> TELTKCKVSHAIKDIDGYQGISLLEWACVLFHTSGYDTQAVVNDNGSTEYGLFQISDRFWCKSSEFPESENICGIS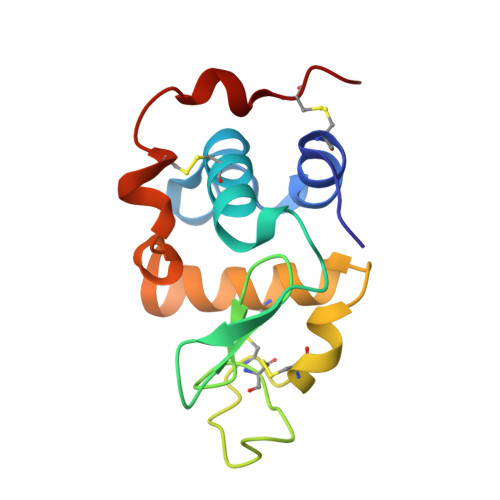CDKLLDDELDDDIACAKKILAIKGIDYWKAYKPMCSEKLEQWRCEKP> MSQIMYNYPAMMAHAGD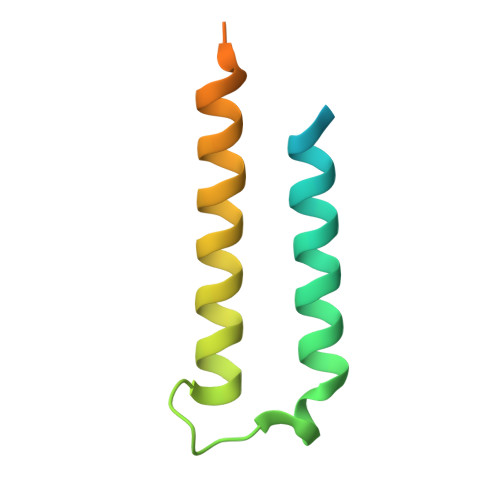MAGYAGTLQSLGADIASEQAVLSSAWQGDTGITYQGWQTQWNQALEDLVRAYQSMSGTHESNTMAMLARDGAEAAKWGG>[2x]LDFQSESYKDAYSRINAIVIEGEQEAFDNYNRLAEMLPDQRDELHKLAKMEQRHMKGFMACGKNLSVTPDMGFAQKFFERLHENFKAAAA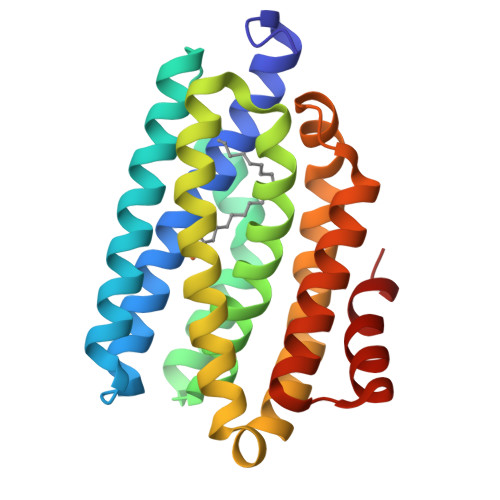EGKVVTCLLIQSLIIECFAIAAYNIYIPVADAFARKITEGVVRDEYLHRNFGEEWLKANFDASKAELEEANRQNLPLVWLMLNEVADDARELGMERESLVEDFMIAYGEALENIGFTTREIMRMSAYGLAAV> AGRFTKVAAAVADSVVT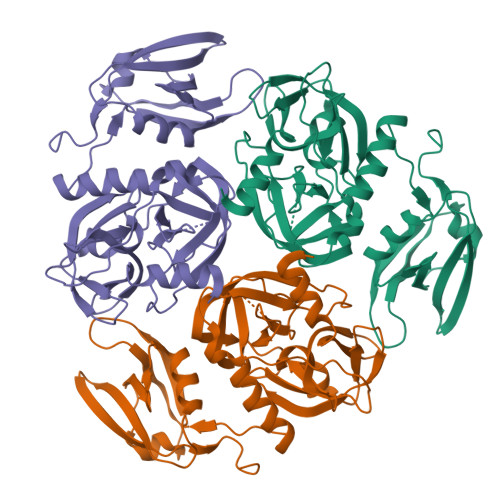IESVSDQEGMQGSGVIVDGRGYIVTNAHVISEAANNPSQFKTTVVFNDGKEVPANLVGRDPKTDLAVLKVDNVDNLTVARLGDSSKVRVGDEVLAVGAPLGLRSTVTQGIVSALHRPVPLSGEGSDTDTVIDAIQTDASINHGNSGGPLIDMDAQVIGINTAGKSLSDSASGLGFAIPVNEMKLVANSLIKDGKIVHPTLGISTRSVSNAIASGAQVANVKAGSPAQKGGILENDVIVKVGNRAVADSDEFVVAVRQLAIGQDAPIEVVREGRHVTLTVKPDPDSTLEH>MELIRIAMKKDLENDNSLMNKWATVAGLKNPNPLYDFLNHDGKTFNEFSSIVNIVKSQYPDREYELMKDYCLNLDVKTKAARSALEYADANMFFEIEDVLIDSMISCSNMKSKEYGKVYKIHRELSNSVITEFEAVKRLGKLNIKTPEMNSFSRLLLLYHYLSTGNFSPMAQLIKQIDLSEISENMYIRNTYQTRVHVLMSNIKLNENSLEECREYSKKALESTNILRFQVFSYLTIGNSLLFSNYELAQENFLKGLSISVQNENYNMIFQQALCFLNNVWRKENKWINFESDSIMDLQEQAHCFINFNENSKAKEVLDKLDLLVHNDNELAMHYYLKGRLEQNKACFYSSIEYFKKSNDKFLIRLPLLELQKMGENQKLLEL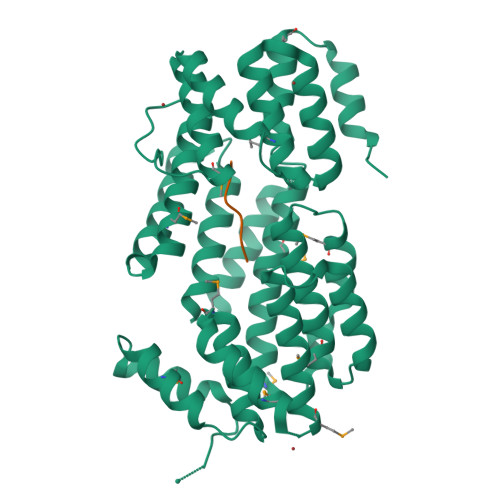LLLLEHHHHHHHH[2x];>GMPRGA[2x]> YAPSALVLTVGKGVSATTAAPERAVTLTCAPGPSGTHPAAGSACADLAAVGGDLNALTRGEDVMCPKVYDPVLLTVDGVWQGKRVSYE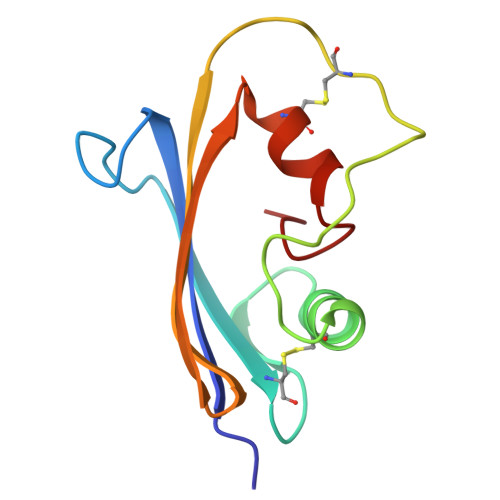RVFSNECEMNAHGSSVFAF> MLRACGVLQLRARPKTVCVEPGSNRLPEALVVEKARDIFGRPEFPGKRVLHNWRFFIKAGKAATGPPVGQEFSKLGLKAMDFAKVFNDRTKPHFKEDVELIVRIQVYFDKS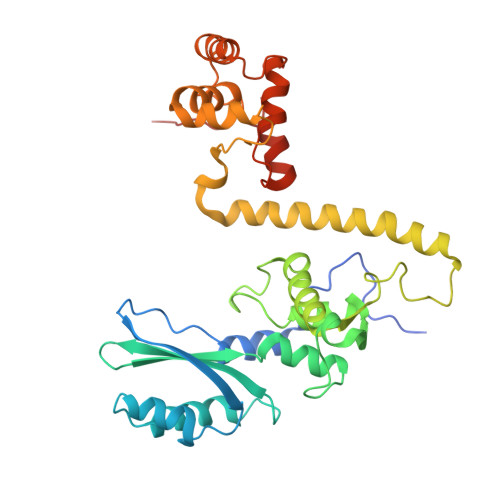YLFTIEPPPTAWFILRALRKKRRETGPVPLRGHYCALMTLEMAYEIAKMKPLCWGRPEYPLLETRVRRVVGQARRMGVCFIGVDTPYSSPVKDMTEQQYTEECERYRRIHMEQYTTLRQRELEEAPLIERLHRPNMSPLTDEQIEEGLRDPCLLDTLWRASHPLSPYHRDLRERELARRYLNARGWVKDMTPEEMRIVFMNYRLPEGEKRKQMDEAAMSGEVYWTRDGAQL>[2x]MGSSHHHHHHSGLVPRGSHMATPPKRSSPSFSASSEGTRIKKISIEGNIAAGKSTFVNILKQLSEDWEVVPEPVARWSNVQSTQD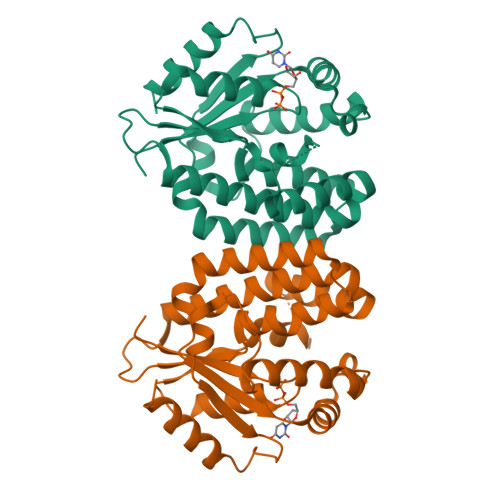EFEELTMEQKNGGNVLQMMYEKPERWSFTFQTYACLSRIRAQLASLNGKLKDAEKPVLFFERSVYSDRYIFASNLYESESMNETEWTIYQDWHDWMNNQFGQSLELDGIIYLQATPETCLHRIYLRGRNEEQGIPLEYLEKLHYKHESWLLHRTLKTNFDYLQEVPILTLDVNEDFKDKYESLVEKVKEFLSTL>MQRLFLLVAVMLLSGCLTAPPKEAARPTLMPRAQSYKDLTHLPAPTGKIFVSVYNIQDETGQFKPYPASNFSTAVPQSATAMLVTALKDSRWFIPLERQGLQNLLNERKIIRAAQENGTVAINNRIPLQSLTAANIMVEGSIIGYESNVKSGGVGARYFGIGADTQYQLDQIAVNLRVVNVSTGEILSSVNTSKTILSYEVQAGVFRFIDYQRLLEGEVGYTSNEPVMLCLMSAIETGVIFLINDGIDRGLWDLQNKAERQNDILVKYRHMSVPPESWSHPQFEK[9x];>[9x]MRVKHAVVLLMLISPLSWAGTMTFQFRNPNFGGNPNNGAFLLNSAQAQNSYKDPSYNDDF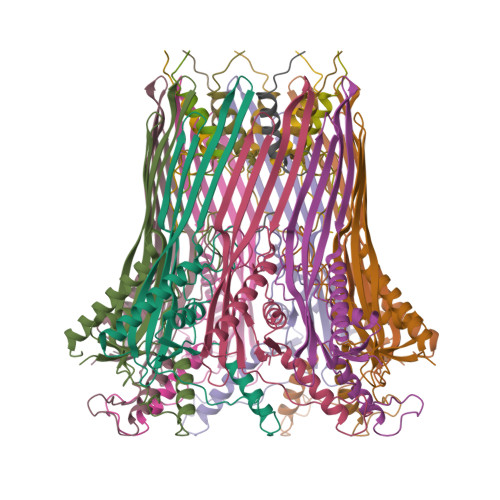GIETPSALDNFTQAIQSQILGGLLSNINTGKPGRMVTNDYIVDIANRDGQLQLNVTDRKTGQTSTIQVSGLQNNSTDFHHHHHH2-(1H-imidazol-1-yl)-9-methoxy-8-(2-methoxyethoxy)benzo[c][2,7]naphthyridin-4-amine | C19 H19 N5 O3 | 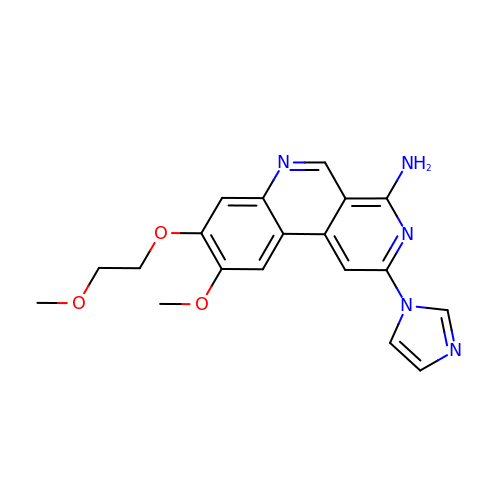QSSGYSRUMIOURP-UHFFFAOYSA-N>[12x]GMTNTTYVQ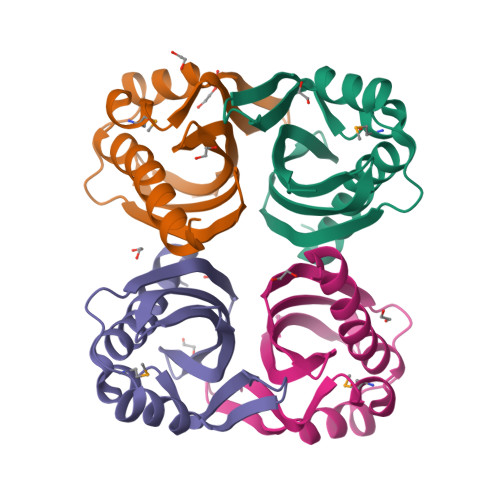EYHAIVEVLSKYNEGGKKADSTIMRPAFSSQATIFGVDVDNKLTGGPIQGLFDVIDNVFHPSPEAKAAIARIDIVGTAASARIDTDDISGFRFTDFFNLLKVEGKWTVVSKIYHTHPSA> M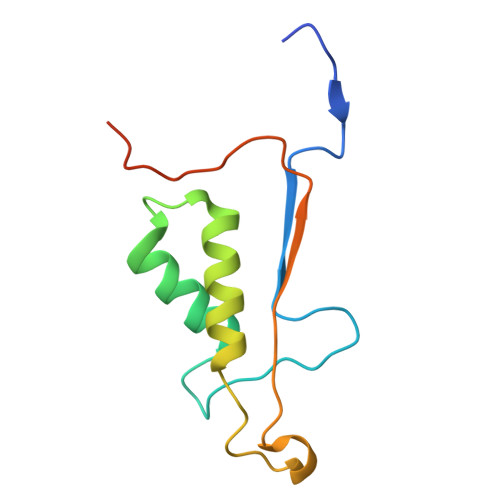AASVYTLPAGADFLMCYSVAEGYYSHRETVNGSWYIQDLCEMLGKYGSSLEFTELLTLVNRKVSQRRVDFCKDPSAIGKKQVPCFASMLTKKLHFFPKSNLEHHHHHH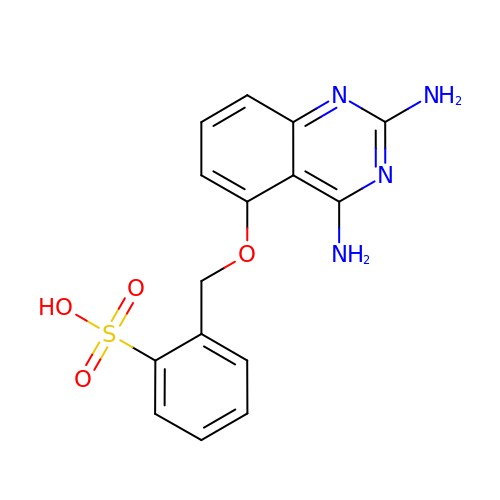2-{[(2,4-diaminoquinazolin-5-yl)oxy]methyl}benzenesulfonic acid | C15 H14 N4 O4 S | RZCCCBZCJSAGMZ-UHFFFAOYSA-N> SDSENLYFQGSQELKSEVFSLLNLDYPGLEKVKALHQEGKDEDAAKALLDYYRARTNVKTPDINLKKITIGKEEQQWADDGLKHTFFVHKGYQPSYNYGEDINWQYWPVKDNELRWQLHRHKWFTPMGKAYRVSGDEKYAKEWAYQYIDWIKKNPLVKMDKKEYELVSDGKIKGEVENVRFAWRPLEVSNRLQDQTTQFQLFLPSPSFTPDFLTEFLVNYHKHAVHILANYSDQGNHLLFEAQRMIYAGAFFPEFKEAPAWRKSGIDILNREVNVQVYNDGGQFELDPHYHLAAINIFCKALGIAD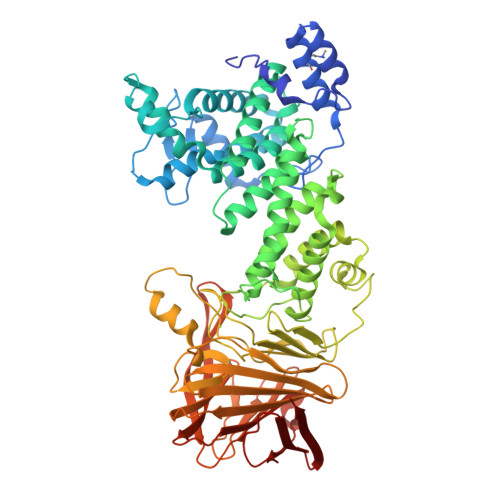VNGFRNEFPQEYLDTIEKMIMFYANISFPDYTNPCFSDAKITEKKEMLKNYRAWSKLFPKNETIKYLATDGKEGALPDYMSKGFLKSGFFVFRNSWGMDATQMVVKAGPKGFWHCQPDNGTFEMWFNGKNLFPDSGSYVYAGEGEVMEQRNWHRQTSVHNTVTLDNKNLETTESVTKLWQPEGNIQTLVTENPSYKNFKHRRSVFFVDNTYFVIVDEVSGSAKGSVNLHYQMPKGEIANSREDMTFLTQFEDGSNMKLQCFGPEGMSMKKEPGWCSTAYRKRYKRMNVSFNVKKDNENAVRYITVIYPVKKSADAPKFDAKFKNKTFDENGLEIEVKVNGKKQSLKYKL> AFSRPGLPVEYLQVPSASMGRDIKVQFQGGGPHAVYLLDGLRAQDDYNGWDINTPAFEEYYQSGLSVIMPVGGQSSFYTDWYQPSQSNGQNYTYKWETFLTREMPAWLQANKGVSPTGNAAVGLSMSGGSALILAAYYPQQFPYAASLSGFLNPSEGWWPTLIGLAMNDSGGYNANSMWGPSSDPAWKRNDPMVQIPRLVANNTRIWVYCGNGTPSDLGGDNIPAKFL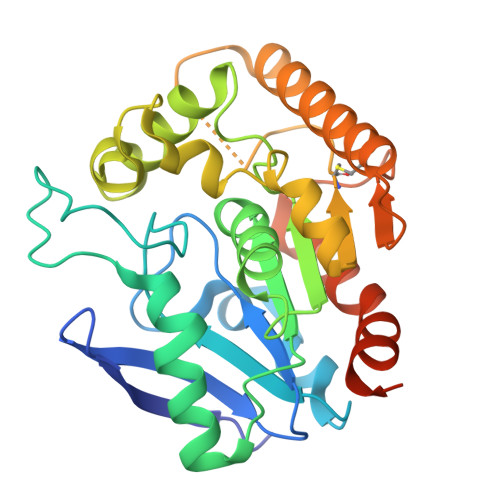EGLTLRTNQTFRDTYAADGGRNGVFNFPPNGTHSWPYWNEQLVAMKADIQHVLNGATPPAAPAAPAAHHHHHH> MTQIIKIDPLNPEIDKIKIAADVIRNGGTVAFPTETVYGLGANAFDGNACLKIFQAKNRPVDNPLIVHIADFNQLFEVAKDIPDKVLEIAQIVWPGPLTFVLKKTERVPKEVTAGLDTVAVRMPAHPIALQLIRESGVPIAAPSANLATRPSPTKAEDVIVDLNGRVDVIIDGGHTFFGVESTIINVTVEPPVLLRPGPFTIEELKKLFGEIVIPEFAQGKKEAEIALAPGMKYKHYAPNTRLLLVENRNIFKDVVSLLSKKYKVALLIPKELSKEFE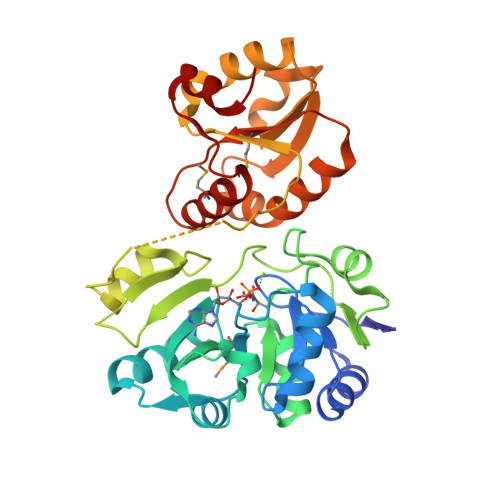GLQQIILGSDENLYEVARNLFDSFRELDKLNVDLGIMIGFPERGIGFAIMNRARKASGFSIIKAISDVYKYVNI>[2x]MAMHPRKDWYELTRATNWTPSYVTEEQLFPERMSGHMGIPLEKWESYDEPYKTSYPEYVSIQREKDAGAYSVKAALERAKIYENSDPGWISTLKSHYGAIAVGEYAAVTGEGRMARFSKAPGNRNMATFGMMDELRHGQLQLFFPHEYCKKDRQFDWAWRAYHSNEWAAIAAKHFFDDIITGRDAISVAIMLTFSFETGFTNMQFLGLAADAAEAGDYTFANLISSIQTDESRHAQQGGPALQLLIENGKREEAQKKVDMAIWRAWRLFAVLTGPVMDYYTPLEDRSQSFKEFMYEWIIGQFERSLIDLGLDKPWYW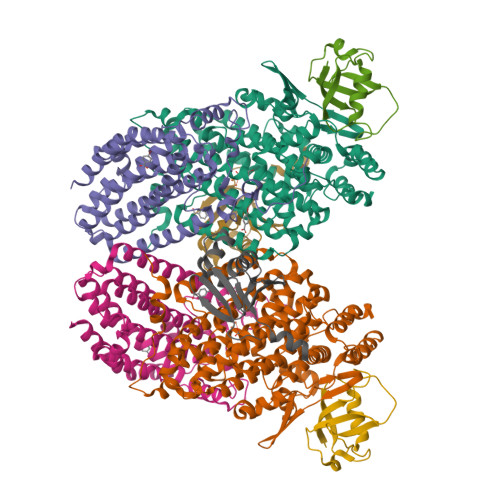DLFLKDIDELHHSYHMGVWYWRTTAWWNPAAGVTPEERDWLEEKYPGWNKRWGRCWDVITENVLNDRMDLVSPETLPSVCNMSQIPLVGVPGDDWNIEVFSLEHNGRLYHFGSEVDRWVFQQDPVQYQNHMNIVDRFLAGQIQPMTLEGALKYMGFQSIEEMGKDAHDFAWADKCKPAMKKSA;>MSFESKKPMRTWSHLAEMRKKPSEYDIVSRKLHYSTNNPDSPWELSPDSPMNLWYKQYRNASPLKHDNWDAFTDPDQLVYRTYNLMQDGQESYVQSLFDQFNEREHDQMVREGWEHTMARCYSPLRYLFHCLQMSSAYVQQMAPASTISNCCILQTADSLRWLTHTAYRTHELSLTYPDAGLGEHERELWEKEPGWQGLRELMEKQLTAFDWGEAFVSLNLVVKPMIVESIFKPLQQQAWENNDTLLPLLIDSQLKDAERHSRWSKALVKHALENPDNHAVIEGWIEKWRPLADRAAEAYLSMLSSD[2x];>MSAFPVHAAFEKDFLVQLVVVDLNDSMDQVAEKVAYHCVNRRVAPREGVMRVRKHRSTELFPRDMTIAESGLNPTEVIDVVFEE[2x];>MSTLADQALHNNNVGPIIRAGDLVEPVIETAEIDNPGKEITVEDRRAYVRIAAEGELILTRKTLEEQLGRPFNMQELEINLASFAGQIQADEDQIRFYFDKTM[2x]6-(trifluoromethyl)pyrimidin-4-amine 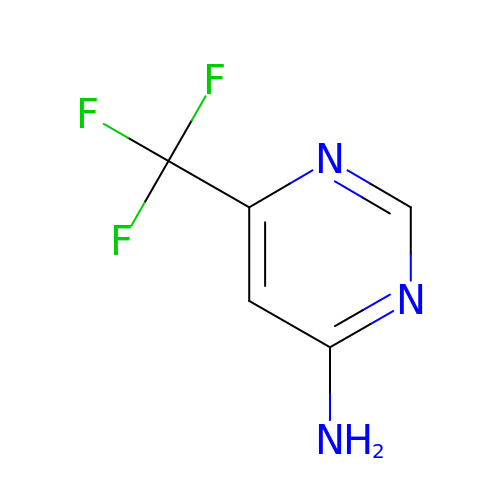| C5 H4 F3 N3 | FIAIKJQZLXLGCR-UHFFFAOYSA-N> G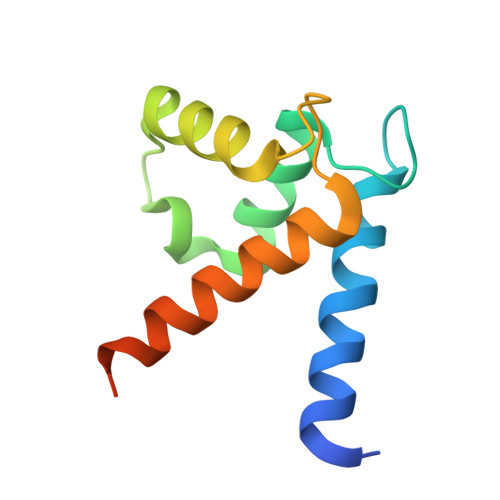SHMACPLEKALDVMVSTFHKYSGKEGDKFKLNKSELKELLTRELPSFLGKRTDEAAFQKLMSNLDSNRDNEVDFQEYCVFLSCIAMMCNEFFEGFPDKQPRKK>MKPDETPMFDPS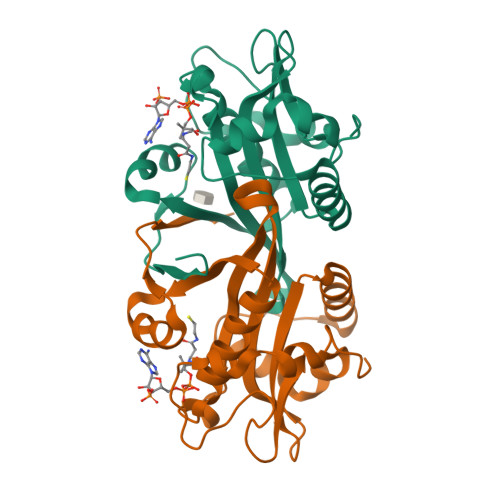LLKEVDWSQNTATFSPAISPTHPGEGLVLRPLCTADLNRGFFKVLGQLTETGVVSPEQFMKSFEHMKKSGDYYVTVVEDVTLGQIVATATLIIEHKFIHSCAKRGRVEDVVVSDECRGKQLGKLLLSTLTLLSKKLNCYKITLECLPQNVGFYKKFGYTVSEENYMCRRFLK[2x]> GMKQIAFIGLGHMGAPMATNLLKAGYLLNVFDLVQSAVDGLVAAGASAARSARDAVQGADVVISMLPASQHVEGLYLDDDGLLAHIAPGTLVLECSTIAPTSARKIHAAARERGLAMLDAPVSGGTAGAAAGTLTFMVGGDAEALEKARPLFEAMGRNIFHAGPDGA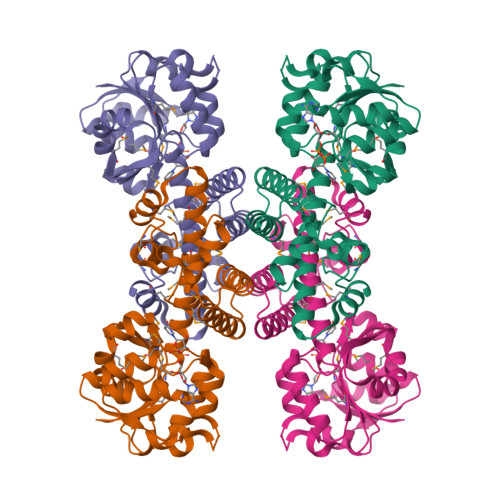GQVAKVCNNQLLAVLMIGTAEAMALGVANGLEAKVLAEIMRRSSGGNWALEVYNPWPGVMENAPASRDYSGGFMAQLMAKDLGLAQEAAQASASSTPMGSLALSLYRLLLKQGYAERDFSVVQKLFDPTQGQ>[2x]MADRIELRGLTVHGRHGVYDHERVAGQRFVIDVTVWIDL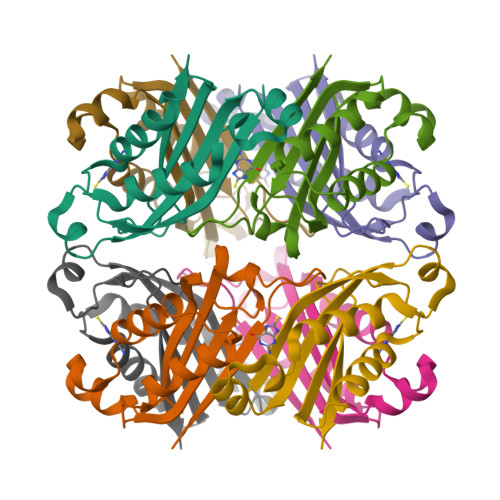AEAANSDDLADTYDYVRLASRAAEIVAGPPRKLIETVGAEIADHVMDDQRVHAVEVAVHKPQAPIPQTFDDVAVVIRRSRRG>[4x]HM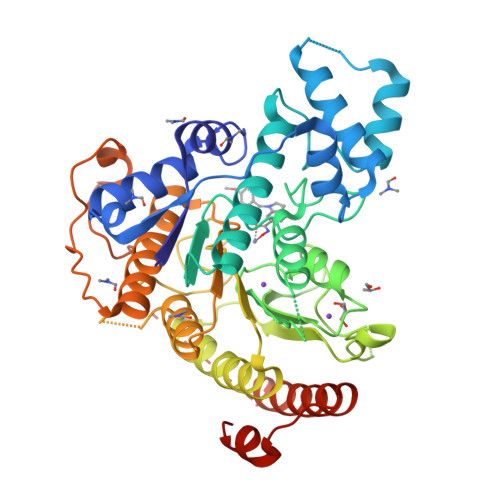SVGIVYGDQYRQLCCSSPKFGDRYALVMDLINAYKLIPELSRVPPLQWDSPSRMYEAVTAFHSTEYVDALKKLQMLHCEEKELTADDELLMDSFSLNYDCPGFPSVFDYSLAAVQGSLAAASALICRHCEVVINWGGGWHHAKRSEASGFCYLNDIVLAIHRLVSSTPPETSPNRQTRVLYVDLDLHHGDGVEEAFWYSPRVVTFSVHHASPGFFPGTGTWNMVDNDKLPIFLNGAGRGRFSAFNLPLEEGINDLDWSNAIGPILDSLNIVIQPSYVVVQCGADCLATDPMRIFRLTNFYPNLNLDSDCDSECSLSGYLYAIKKILSWKVPTLILGGGGYNFPDTARLWTRVTALTIEEVKGKKMTISPEIPEHSYFSRYGPDFELDIDYFPHESHNKTLDSIQKHHRRILEQLRNYADLNKLIYDYDQVYQLYNLTGMGSLVPR TSG-6 is a 35-kDa (single chain) protein composed mainly of contiguous Link and CUB modules that are flanked by N- and C-terminal sequences of 18 and 29 amino acids, respectively. TSG-6 was shown to play a direct role in the transfer of HCs from IαI onto HA via the formation of covalent intermediates (HC1·TSG-6 and HC2·TSG-6) and act as a catalyst in this process. Hyaluronan is organized into a cross-linked network by the cooperative action of three proteins, inter-α-inhibitor (IαI), pentraxin-3, and TNF-stimulated gene-6 (TSG-6), driving the expansion of the COC and providing the cumulus matrix with its required viscoelastic properties. Here, we have determined the tertiary structure of the CUB module from human TSG-6, identifying a calcium ion-binding site and chelating glutamic acid residue that mediate the formation of HC·TSG-6.

To test our prediction that a functionally important metal ion-binding site is present within human TSG-6 (37, 85), we determined the crystal structure of its CUB module to 2.3 Å; this was based on the crystallization of the human CUB_C domain (i.e. the CUB module and the C-terminal 29 amino acid residues), which we had previously shown by NMR spectroscopy to be folded. This revealed it to have a classical CUB-type jelly roll fold, with a greater degree of similarity to the metal ion-binding subclass of CUB domains (C1s, MASPs) compared with the non-metal ion-binding spermadhesins, and, consistent with this, it contained a divalent cation at the site we had predicted. The metal ion-binding site in the TSG-6 CUB module consists of seven oxygen ligands with pentagonal bipyramidal coordination geometry. This is composed of the main chain carbonyl groups of Ser-234 and Val-235, monodenate coordination with side chain carboxylate groups of Glu-183 and Asp-232, and bidentate coordination with the carboxylate of Asp-191 and a buried water molecule, an arrangement highly suggestive of Ca2+ (or perhaps Mn2+). However, no magnesium ion-binding sites were discovered during the refinement and analysis of the TSG-6 CUB module structure, despite the presence of 200 mm MgSO4 in the crystallization conditions. Overall, these data provide evidence that Ca2+ is not required for stabilization of the TSG-6 CUB module fold but rather plays a role in the local organization of loops surrounding the calcium ion-binding site and perhaps also has some effect on the stability of the protein core. The Glu-183 residue, which is involved in chelating the Ca2+ ion, makes a major contribution to the non-covalent interaction with HCs of IαI (e.g. via their Mg2+-containing MIDAS motifs), which precedes formation of the covalent bond between TSG-6 and HC. In particular, it probably orients the functionally important Glu-183 amino acid residue, allowing it to interact with the HC.

> NPHAKECGGVFTDPKQIFKSPGFPNEYEDNQICYWHIRLKYGQRIHLSFLDFDLEDDPGCLADYVEIYDSYDDVHGFVGRYCGDELPDDIISTGNVMTLKFLSDASVTAGGFQIKYVAMDPVSKSSQGKNTSTTSTGNKNFLAGRFSHL3-methyl-6-[[(1-methylcyclopropyl)amino]-bis(oxidanyl)-$l^{4}-sulfanyl]-1-(phenylmethyl)quinazoline-2,4-dione | C20 H23 N3 O4 S 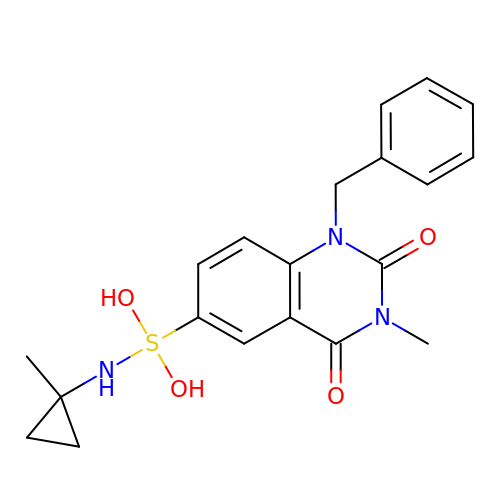| WQSNZLBPHUSAAJ-UHFFFAOYSA-N> MSFVDHPPDWLEEVGEGLREFLGLEAGPPKPKPNQQHQDQARGLVLPGYNYLGPGNGLDRGEPVNRADEVAREHDISYNEQLEAGDNPYLKYNHADAEFQEKLADDTSFGGNLGKAVFQAKKRVLEPFGLVEEGAKTAPTGKRIDDHFPKRKKARTEEDSKPSTSSDAEAGPSGSQQLQIPAQPASSLGADTMSAGGGGPLGDNNQGADGVGNASGDWHCDSTWMGDRVVTKSTRTWVLPSYNNHQYREIKSGSVDGSNANAYFGYSTPWGYFDFNRFHSHWSPRDWQRLINNYWGFRPRSLRVKIFNIQVKEVTVQDSTTTIANNLTSTVQVFTDDDYQLPYVVGNGTEGCLPAFPPQVFTLPQYGYATLNRDNGDNPTERSSFFCLEYFPSKMLRTGNNFEFTYSFEEVPFHCSFAPSQNLFKLANPLVDQYLYRFVSTSATGAIQFQKNLAGRYANTYKNWFPGPMGRTQGWNTSSGSSTNRVSVNNFSVSNRMNLEGASYQVNPQPNGMTNTLQGSNRYALENTMIFNAQNATPGTTSVYPEDNLLLTSESETQPVNRVAYNTGGQMATNAQNATTAPTVGTYNLQEVLPGSVWMERDVYLQGPIWAKIPETGAHFHPSPAMGGFGLKHPPPMMLIKNTPVPGNITSFSDVPVSSFITQYSTGQVTVEMEWELKKENSKRWNPEIQYTNNYNDPQFVDFAPDGSGEYRTTRAIGTRYLTRPL;> MASVSAGESVQITLPKNEVQLNAYVLQEPPKGETYTYDWQLITHPRDYSGEMEGKHSQILKLSKLTPGLYEFKVIVEGQNAHGEGYVNVTVKPEPRKNRPPIAIVSPQFQEISLPTTSTVIDGSQSTDDDKIVQYHWEELKGPLREEKISEDTAILKLSKLVPGNYTFSLTVVDSDGATNSTTANLTVNKAVDYPPVANAGPNQVITLPQNSITLFGNQSTDDHGITSYEWSLSPSSKGKVVEMQGVRTPTLQLSAMQEGDYTYQLTVTDTIGQQATAQVTVIVQPENNK

Adeno-associated virus (AAV) is a small ssDNA satellite virus of high interest (in recombinant form) as a safe and effective gene therapy vector. AAV’s human cell entry receptor (AAVR) contains polycystic kidney disease (PKD) domains bound by AAV. Seeking understanding of the spectrum of interactions, goat AAVGo.1 is investigated, because its host is the species most distant from human with reciprocal cross-species cell susceptibility. The AAV5 clade also includes AAVGo.1 (18, 19), which was isolated from deceased neonatal domesticated goat ileum.

The AAVGo.1 cryo-EM structure of a complex with a PKD12 fragment of AAVR at 2.4 Å resolution shows PKD1 bound with minimal change in virus structure. Just PKD1 was observed in the AAVGo.1 complex, with the two-domain PKD12 cryo-EM reconstruction and receptor density for the PKD1 subunit strongest at the viral interface. There are only minor conformational adaptations in AAVR, but there is a near-rigid rotation of PKD1 with maximal displacement of the receptor domain by ~1 Å compared to PKD1 bound to AAV5. Displacements of ~1 Å are observed between PKD1 backbone carbons, and the shift appears to be a rotation around Arg353 that remains essentially unmoved. The complex of AAVGo.1 bound to PKD12 differed in modest ways at the VR-VII and VR-IX interfaces. In AAVGo.1, however, these residues are replaced by Ser442 and Ala443, and interactions with PKD1 Lys399 are absent. Therefore, AAV5 VR-IV has unique contacts with the PKD1 C terminus absent in the AAVGo.1-PKD1 complex. The AAV5 VR-VII residue Gln532 makes contact with PKD1 (Ile349), and the Ile349 interaction is absent in AAVGo.1. The lysine can be modeled within the density for Arg353 in the map of the AAVGo.1-PKD12 receptor complex, suggesting that goat AAVR might be only minimally different and that Lys353 might have interactions similar to what we observe with human PKD1 Arg353 in the AAVGo.1 binding pocket. At first approximation, the binding of AAVGo.1 to AAVR is similar to that of AAV5, so the one exception becomes a second structural class in terms of the mode of binding.>GCDDDPVLLKDPVSALSNDCIKRSLPVAPNIVGNEIEFAYAMAIPNELGKLSSAQVVSSIAGATGTYFDPNSYYTNSSGQDIPVKVCSDSQTNGTTTVIDFTVDTCAATLRYYYIIPEEARGKDVQFSFSVKASNGQVAEYKLGPYKISKMDMAKNLSVTNDKCYLSFLNEGEAVHIYSKADLQANPSLAAKIDIMYAYSEKSDLSHAFYTSSSPKEYMGGTELPSGFVNNTKMIKVYGLQDRQLSDLQYSKFIDDLDFETIDMSKCTNYILGLKEEAGAWVETADGKYRAYVYINKASAS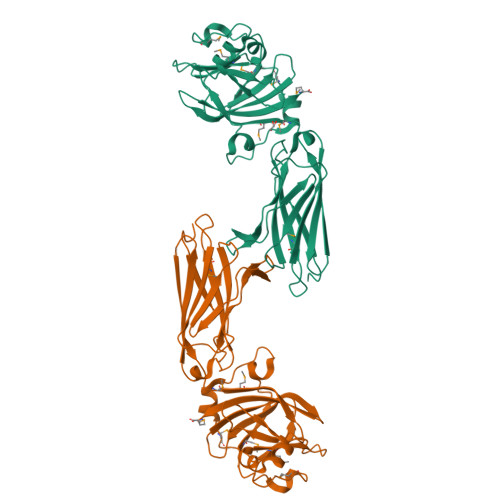EVTVSVKRYKM[2x]The S. marcescens Rap proteins represent founder members of a new bacterial protein family, members of which represent immunity proteins for T6-secreted toxins, as exemplified by Rap1a and Rap2a. We have determined the structures of two members of this family, Rap1b and Rap2b, revealing a new protein fold. The Rap subunit is constructed around a helical bundle of five helices (α2–α6). The Rap proteins display an extensive dimerization interface, consistent with the observation that each Rap protein exists as a stable dimer in solution.

Well-ordered crystals of Rap1b and Rap2b were obtained and the structures were elucidated at 1.9 Å and 2.0 Å resolution respectively. Rap2b has two dimers, formed by subunits A : B and C : D, in the asymmetric unit. The four subunits are similar, with the root-mean-square deviation (r.m.s.d.) between superimposed Cα atoms ranging from 0.5 Å (subunit B and D) to 0.7 Å (subunits A and C). An overlay of Rap1b and Rap2b subunits matches 71 Cα atoms with a r.m.s.d. of 1.4 Å. A disulphide linkage (Cys54–Cys120 in Rap1b, Cys41–Cys101 in Rap2b) tethers α2 and α5 together. The Rap1b dimer uses almost 24% of the accessible surface area of a subunit in formation of the dimer. In the case of Rap2b the value is 20%. Surprisingly for proteins with such low pI values, the striking surface feature conserved in Rap1b and Rap2b structures is a crescent-shaped basic patch on either side of the dimer. It is possible that such a basic crescent, if present on toxin-binding Rap proteins, may contribute to orientation of the partner during binding; conversely, it might contribute to the lack of Ssp binding by Rap1b and Rap2b. Additionally, Rap2b shares slightly higher sequence identity with Rap2a (23% identity for the mature proteins) than it does with Rap1b (20% identity).

>[4x]GHMENSLNALSQEALYKNWLTSRCIGKSTDSERTKQDAFRSASAYLELSKLPMDAFEQGEKLAEQYANKNSQGSVQGTYHTLDCLSLQNASEAETIFERYSK> KYKALAREAALSKIGELASEIFAEFTEGKYSEVVVRAEENKVRLFVVWEGKERPLTFLSGGERIALGLAFRLAMSLYLAGEISLLILDE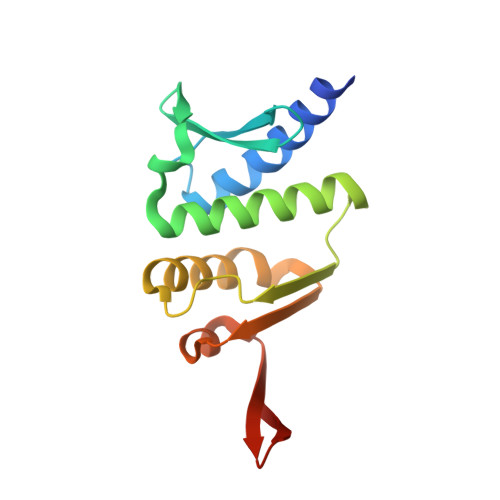PTPYLDEERRRKLITIMERYLKKIPQVILVSHDEELKDAADHVIRISLENGSSKVEVVS tert-butyl 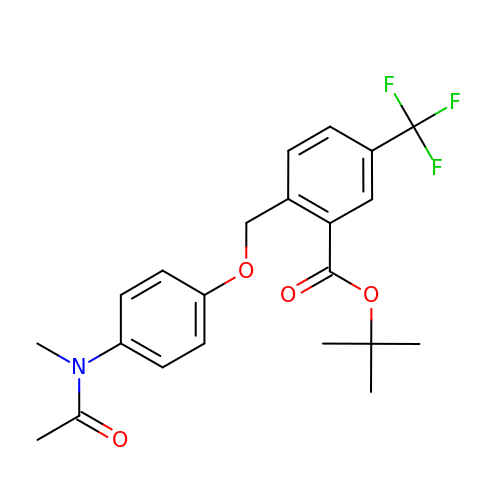2-[[4-[ethanoyl(methyl)amino]phenoxy]methyl]-5-(trifluoromethyl)benzoate | C22 H24 F3 N O4 | YZWZMPWHXSZLBQ-UHFFFAOYSA-N(2,5-dimethyl-1,3-thiazol-4-yl)(pyrrolidin-1-yl)methanone | C10 H14 N2 O S | 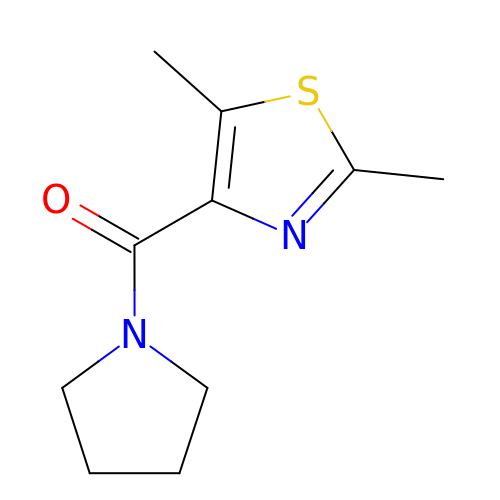BRAPKXFMPGACJU-UHFFFAOYSA-N>[4x]GGAAGGCCGAAAGGUC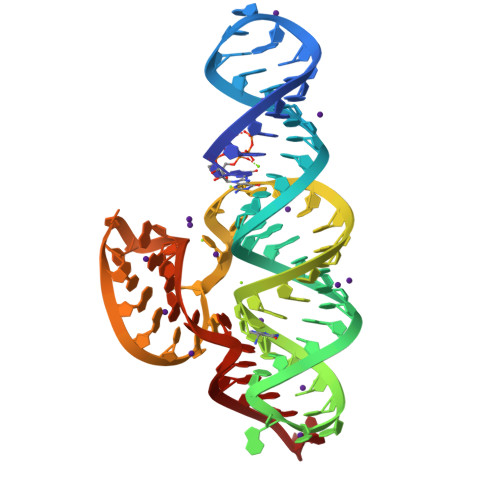UUCCACGACGAUACUUAUUUCCUUUGAUCGUCGUUAUUACUGGCUUCGGCCACAAAGGAGA>CGAATTCG[2x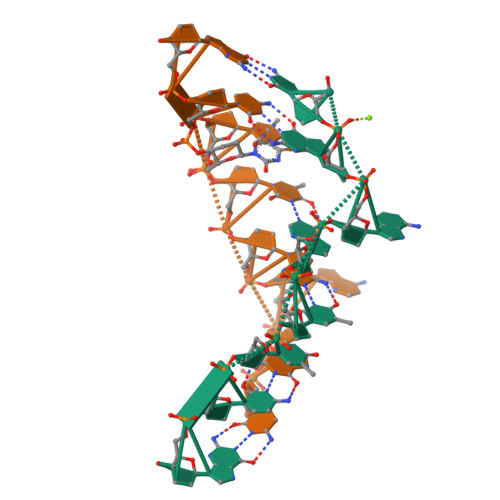]> MAGIFDRIAGASGADETELTAEPMALDDGMDGEQPAMSANIQVDERRTPQRVREAVQEMLKYGLLEESHKPNLYRSALTNIEVVDRILEPLDLAMGVDEVRGLVFVTVRQGEVAEQDDWSHPLVRRQRLNLEQSLLIAILRQHFIAYEQESGTGASQALVAVDELIPQLQVYLGELGSEAKERNRIITLLDQLKGHGLVSALDAHDRV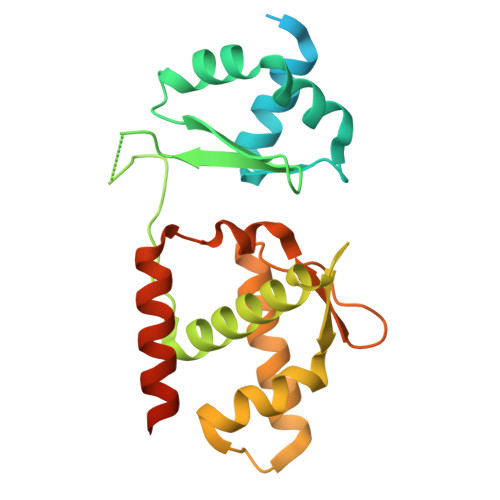IIRPIITHLANPENLQALVVWLREQVEGAVTPAAGGEEDEA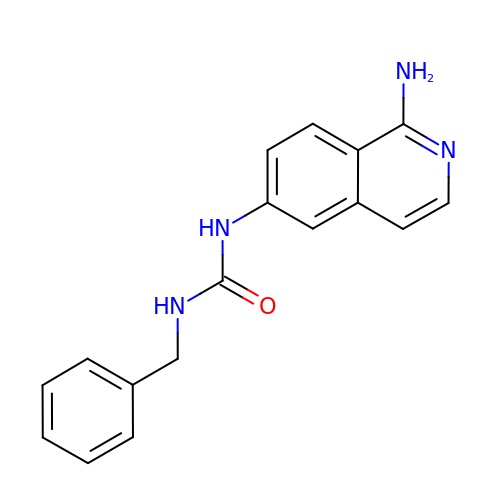1-(1-azanylisoquinolin-6-yl)-3-(phenylmethyl)urea | C17 H16 N4 O | HFHRTXJNMUTIEE-UHFFFAOYSA-N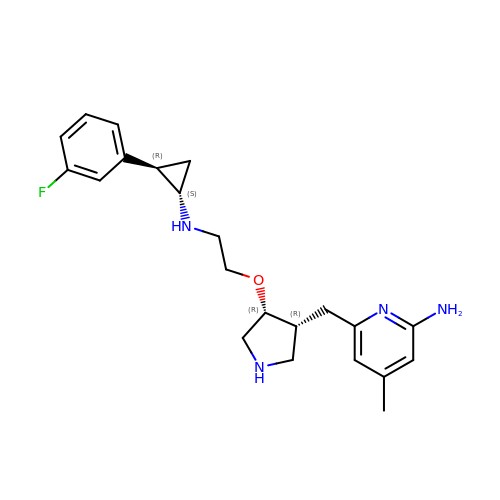6-{[(3R,4R)-4-(2-{[(1S,2R)-2-(3-fluorophenyl)cyclopropyl]amino}ethoxy)pyrrolidin-3-yl]methyl}-4-methylpyridin-2-amine | C22 H29 F N4 O | OPKCBCPSRYBLIJ-DBOLQNLKSA-N>SMTDLLSAEDIKKAIGAFTAADSFDHKKFFQMVGLKKKSADDVKKVFHILDKDKSGFIEEDELGSILKGFSSDARDLSAKETKTLMAAGDKDGDGKIGVEEFSTL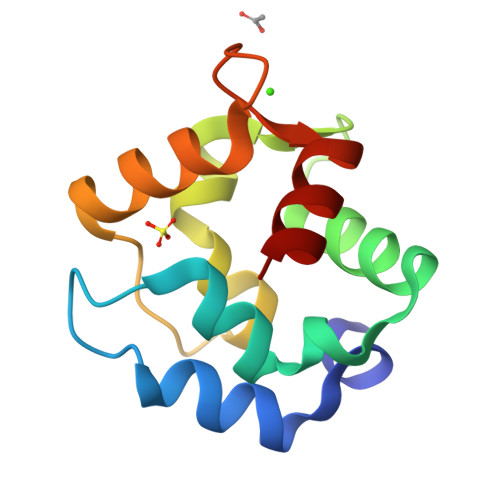VAES[3x]> GVTPPQITAQTYVLMDYNSGAILTALNPDQRQYPASLTKMMTSYVVGVALKQGKIHNTDMVTIGESAWGRNFPDSSKMFLDLNTQVSVADLNRGVIVVSGNDATVALAEHISGNVPNFVETMNKYVQQFGLKNTNFTTPHGLDDPNQYSSARDMAIIGAHIIRDLPEEYKIYSEKDFTFNKIKQPNRNGLLWDKTINVDGMKTGHTSQAGYNLVASATTSNNMRLISVVMGVPTYKGREVESKKLLQWGFANFETFKTLEAGKEISEQRVY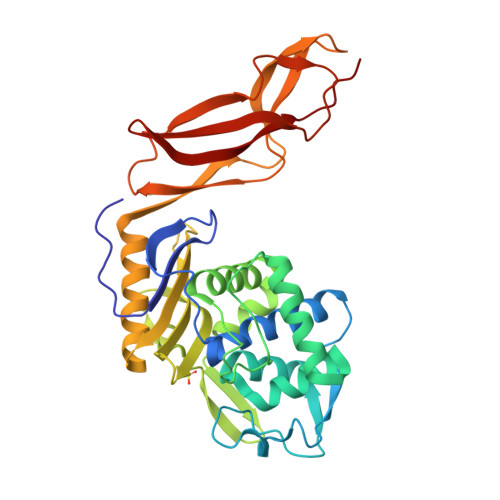YGDKNSVKLGAFMDHFITIPKGKQSEVKARYELADKNLQAPLAKGQVIGKVVYALDGKDIASANLQVMNDVGE> MGESERSEAFGIPRDSPLSSGDAAELEQLRREAAVLREQLENAVGSHAPTRSARDIHQLEARIDSLAARNSKLMETLKEARQQLLALREEVDRLGQPPSGYGVLLATHDDDTVDVFTSGRKMRLTCSPNIDAASLKKGQTVRLNEALTVVEAGTFEAVGEISTLREILADGHRALVVGHADEERVVWLADPLIAEDLPDGLPEALNDDTRPRKLRPGDSLLVDTKAGYAFERIPKAEVEDLVLEEVPDVSYADIGGLSRQIEQIRDAVELPFLHKELYREYSLRPPKGVL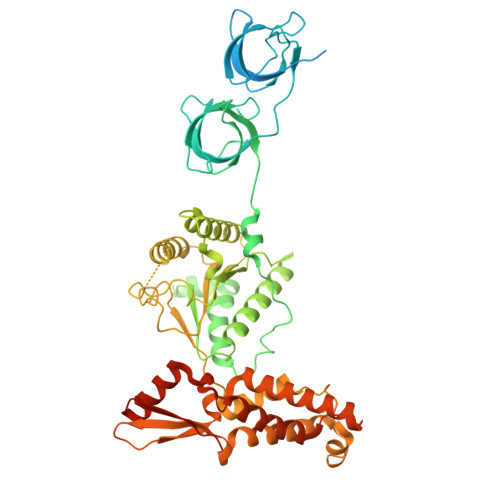LYGPPGCGKTLIAKAVANSLAKKMAEVRGDDAHEAKSYFLNIKGPELLNKFVGETERHIRLIFQRAREKASEGTPVIVFFDEMDSIFRTRGTGVSSDVETTVVPQLLSEIDGVEGLENVIVIGASNREDMIDPAILRPGRLDVKIKIERPDAEAAQDIYSKYLTEFLPVHADDLAEFDGDRSACIKAMIEKVVDRMYAEIDDNRFLEVTYANGDKEVMYFKDFNSGAMIQNVVDRAKKNAIKSVLETGQPGLRIQHLLDSIVDEFAENEDLPNTTNPDDWARISGKKGERIVYIRTLVTGKSSSASRAIDTESNLGQYL> SRFSGQRDHDAVDEFINAVETYKEVEGISDKDALKGLPLLFKSIAVVWWKGVRRDAKTWSDALQLLRDHFSPT

One of the key proteins in long-term synaptic plasticity and memory is the activity-regulated cytoskeleton-associated protein (Arc). Drosophila has two isoforms of Arc, dArc1 and dArc2, with low sequence similarity to mammalian Arc, but lacking a large N-terminal domain. Both dArc isoforms are related to the Ty3/gypsy retrotransposon capsid, consisting of N- and C-terminal lobes. As opposed to the corresponding mammalian Arc lobe domains, which are monomeric, the dArc lobes were all oligomeric in solution, indicating a strong propensity for homophilic interactions.

In our 1.90-Å crystal structure, dArc2-NL is a domain-swapped dimer, in which the second and third helix of the canonical lobe domain join to form an extended helix. One layer of the dimer is formed by α2 of each subunit, which pack at a cross angle of 140.7°. The other layer is formed by the remaining helices, and α1 lies in a groove formed between α2 and α3. The subunit interface of the dimer spans 3440 Å2 of buried surface area. The interface consists exclusively of π-π and van der Waals interactions, and the helices encapsulate a hydrophobic core between the monomers, formed by Phe51, Val55, Pro74, Phe77, Ile80, Trp84, Trp95, Leu99, Leu102, and Phe106. The solvent-exposed surface of the dimer is charged and polarized; the electrostatic surface potential of the side formed by the two coiled α2 helices is highly positive, while the opposite surface formed by α1 and α3 is mainly negative. Only a part of the tail (residues 37–45) was included in the dArc2-NL crystallized here, reflecting the fact that our experiments were carried out before structural information for the capsids and the importance of the N-terminal tail was available. In our structure, this fragment could not be resolved, due to flexibility. The binding surface for the N-terminal segment is buried at the interface of the dArc2-NL domain-swapped dimer. Taken together, the structure of dArc2-NL reveals an intrinsic property of the Arc lobe domain to form alternate dimers via domain swapping, possibly regulated through interactions of the folded dArc2-NL core domain with the N-terminal tail.>MAAACRSVKGLVAVITGGASGLGLATAERLVGQGASAVLLDLPNSGGEAQAKKLGNNCVFAPADVTSEKDVQTALALAKGKFGRVDVAVNCAGIAVASKTYNLKKGQTHTLEDFQRVLDVNLMGTFNVIRLVAGEMGQNEPDQGGQRGVIINTASVAAFEGQVGQAAYSASKGGIVGMTLPIARDLAPIGIRVMTIAPGLFGTPLLTSLPEKVCNFLASQVPFPSRLGDPAEYAHLVQAIIENPFLNGEVIRLDGAIRMQP[4x];> MKSSVQEECVSTISSSKDEDPLAATREFIEMWRLLGREVPEHITEEELKTLMECVSNTAKKKYLKYLYTKEKVKKARQIKKEMKAAAREEAKNIKLLETTEEDKQKNFLFLRLWDRNMDIAMGWKGAQAMQFGQPLVFDMAYENYMKRKELQNTVSQLLESEGWNRRNVDPFHIYFCNLKIDGALHRELVKRYQEKWDKLLLTSTEKSHVDLFPKDSIIYLTADSPNVMTTFRHDKVYVIGSFVDKSMQPGTSLAKAKRLNLATECLPLDKYLQWEIGNKNLTLDQMIRILLCLKNNGNWQEALQFVPKRKHTGFLEISQHSQEFINRLKKAKTAENLYFQSHHHHHHDYKDDDDK

Here, we present several cryo-EM structures of the mitochondrial RNase Z complex (ELAC2/SDR5C1/TRMT10C) bound to different maturation states of mitochondrial tRNAHis, showing the molecular basis for tRNA-substrate selection and catalysis. The human long form of RNase Z, ELAC2, has two alternative start codons to produce a nuclear and a mitochondrially targeted form. TRMT10C is a purine N1-methyltransferase that acts at position 9 of mt-tRNAs using S-adenosylmethionine (SAM) as a co-substrate. SDR5C1 is a moonlighting homotetrameric short-chain dehydrogenase/reductase.

The TRMT10C/SDR5C1 platform in the RNase Z-HCCA complex is similar to the RNase Z-HS and RNase ZH548A-HS complexes, but here, ELAC2 pivots by ~6 degrees around the tRNA (Fig. EV3A). Within the complex, a tetramer of SDR5C1 forms a flat platform that can be bound from each flat side by TRMT10C and precursor mt-tRNA. Thus, the SDR5C1/TRMT10C subcomplex can support the simultaneous processing of two tRNA molecules. Furthermore, the structure shows how TRMT10C compensates for the lack of strong D arm/T arm interactions in most bilaterian mitochondrial tRNAs by providing structural support through its extensive interactions with the mt-tRNA’s D arm. In addition, TRMT10C’s N-terminal domain stabilizes the T loop via electrostatic interactions with the RNA backbone. Here, the structures show that the NTD of TRMT10C binds to the tRNA T loop to stabilize its fold and facilitate the tRNA interaction with the ELAC2 exosite.>GAMATEQIQHIAIVGSVHGKYREMYRQLSEYEKSTGKEISFVICTGDMQTLRYEADLVYLKVPPKYKQMGDFHLYYEGKEKAPYLTLFIGGNHESSNVLLHLYNGGFVCFNMYYLGVCSCININGLRIVGVSGIYKSFDEKKPYTYPPSPNDVVSLFHTRNYVIQMLSNLSQSSQIDISLSHDWPQGIVMKGNYKQLYRFQPGFKKDGASLGSPINKVILNTLKPKYWISGHMHCEYHAEEGPTHFIALGKIGYKNAISYLDLPLKQKTDLEYDKDWVCNLIMTWPAFSNKAQFPDLSYSISELLSKRTKELDKKIIELWEKYIGLKIIYDSDTFDIQFTSRRFYIEKIYNELNIN[5x]

The spliceosome excises introns from nascent messenger RNA (1) in the form of a lariat containing an unusual 2′,5′-phosphodiester linkage (2). Hydrolysis of this linkage is rate-limiting in lariat degradation after splicing, and is required for efficient maturation of many small nucleolar RNAs (snoRNA) and micro RNAs (mirtrons) that are derived from intronic RNA. Dbr1 is tuned to hydrolyze 2′,5′-phosphodiester RNA linkages in branched RNA and not the considerably more abundant canonical 3′,5′-phosphodiester linkages, although the molecular basis for this selectivity has remained elusive for several decades despite extensive biochemical characterization of the enzyme. Sequence analyses predict Dbr1 consists of an N-terminal domain belonging to the metallophosphoesterase (MPE) superfamily of enzymes and a C-terminal domain (CTD) lacking detectible sequence similarity to any other class of protein.

The α pocket cysteine of Dbr1 was substituted to serine to prevent hydrolysis of larger RNA substrate analogs, such as AK65, a synthetic, linear RNA that possesses the 2′ phosphate at the conserved branchpoint adenosine but lacks the 2′ nucleotide that would be present in the complete lariat branchpoint. The structure of the AK65•Dbr1(C14S) complex shows that the enzyme engages the branchpoint nucleotide in a C2′-endo conformation that, in concert with stacking of the adenine base between His16 and Tyr64, places the pseudo-equatorial 2′ phosphate adjacent to the metal binding center and within hydrogen bonding distance of Asn90 and His91. There are few sequence-specific protein-RNA interactions at the branchpoint, consistent with the need for Dbr1 to hydrolyze lariat RNAs containing atypical branchpoint nucleotides. However, a pyrimidine is predicted to be suboptimal for aromatic stacking with His16 and Tyr64, consistent with the reduced activity observed toward cytidine branchpoints. Conversely, substitution by guanosine could promote tighter binding of the branchpoint nucleotide through hydrogen bonding interactions between N1 and N2 and the side chain of Gln47. The structure also demonstrates that the LRL element unique to Dbr1 enzymes acts as a recognition module, with five of its residues (Ile132, Lys134, Phe136, Phe155 and His156) engaging the single-stranded arm 3′ to the branchpoint adenosine. The interactions between RNA and the LRL are stabilized by secondary contacts between the LRL and the CTD involving residues 141–144 and 290–293, respectively. In the other three AK65•Dbr1 complexes in the asymmetric unit, the 5′ nucleotide is disordered and not visible in the electron density maps. Thus, Dbr1 does not appear to recognize nucleotides 5′ to the branchpoint, but instead recognizes the branchpoint and flanking nucleotides directly and utilizes base stacking interactions between the 2′ and 3′ nucleotides to further stabilize the complex.> MDGVHDLAGVQGFGKVPHTVNADIGPTFHAEWEHLPYSLMFAGVAELGAFSVDEVRYVVERMEPRHYMMTPYYERYVIGVATLMVEKGILTQDELESLAGGPFPLSRPSESEGRPAPVETTTFEVGQRVRVRDEYVPGHIRMPAYCRGRVGTISHRTTEKWPFPDAIGHGRNDAGEEPTYHVKFAAEELFGSDTDGGSVVVD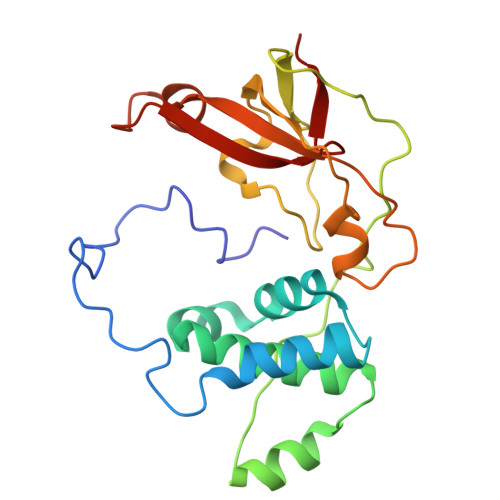LFEGYLEPAA> MKTVGYAIVGTGYFGAELGRIMKEQEGARIVAVLDPENGQTIAEELDCDVETDLDTLYSREDVEAVIVATPNYLHKEPVIKAAEHGVNVFCEKPIALSYQDCDEMVRTCQEHGVIFMAGHVMNFFHGVRYAKKLINDGVIGKVLYCHSARNGWEEQQPTISWKKIREKSGGHLYHHIHELDCVQFLMGGMPEEVTMTGGNVAHQGEAFGDEDDMLFVNMQFSDNRYAVLEWGSAFH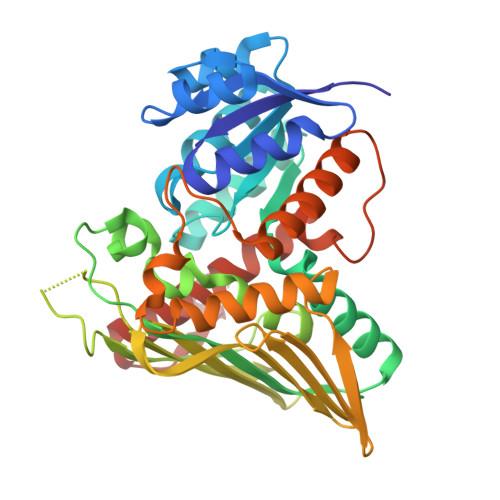WPEHYVLIQGTKGAIKIDMCDCGGTLKVDGREEHFLVHESQEEDDDRTRIYHGTEMDGAIMYGKPGKKPPMWLHSIMKNEMKYLNGILHGKEVDDEFRPLLTGEAARAAIATADACTKSRFEDRKVKLSEIIG>MEPHVLGAVLYWLLLPCALLAACLLRFSGLSLVYLLFLLLLPWFPGPTRCGLQGHTGRLLRALLGLSLLFLVAHLALQICLHIVPRLDQLLGPSCSRWETLSRHIGVTRLDLKDIPNAIRLVAPDLGILVVSSVCLGICGRLARNTRQSPHPRELDDDERDVDASPTAGLQEAATLAPTRRSRLAARFRVTAHWLLVAAGRVLAVTLLALAGIAHPSALSSVYLLLFLALCTWWACHFPISTRGFSRLCVAVGCFGAGHLICLYCYQMPLAQALLPPAGIWARVLGLKDFVGPTNCSSPHALVLNTGLDWPVYASPGVLLLLCYATASLRKLRAYRPSGQRKEAAKGYEARELELAELDQWPQERESDQHVVPTAPDTEADNCIVHELTGQSSVLRRPVRPKRAEPREASPLHSLGHLIMDQSYVCALIAMMVWSITYHSWLTFVLLLWACLIWTVRSRHQLAMLCSPCILLYGMTLCCLRYVWAMDLRPELPTTLGPVSLRQLGLEHTRYPCLDLGAMLLYTLTFWLLLRQFVKEKLLKWAESPAALTEVTVADTEPTRTQTLLQSLGELVKGVYAKYWIYVCAGMFIVVSFAGRLVVYKIVYMFLFLLCLTLFQVYYSLWRKLLKAFWWLVVAYTMLVLIAVYTFQFQDFPAYWRNLTGFTDEQLGDLGLEQFSVSELFSSILVPGFFLLACILQLHYFHRPFMQLTDMEHVSLPGTRLPRWAHRQDAVSGTPLLREEQQEHQQQQQEEEEEEEDSRDEGLGVATPHQATQVPEGAAKWGLVAERLLELAAGFSDVLSRVQVFLRRLLELHVFKLVALYTVWVALKEVSVMNLLLVVLWAFALPYPRFRPMASCLSTVWTCVIIVCKMLYQLKVVNPQEYSSNCTEPFPNSTNLLPTEISQSLLYRGPVDPANWFGVRKGFPNLGYIQNHLQVLLLLVFEAIVYRRQEHYRRQHQLAPLPAQAVFASGTRQQLDQDLLGCLKYFINFFFYKFGLEICFLMAVNVIGQRMNFLVTLHGCWLVAILTRRHRQAIARLWPNYCLFLALFLLYQYLLCLGMPPALCIDYPWRWSRAVPMNSALIKWLYLPDFFRAPNSTNLISDFLLLLCASQQWQVFSAERTEEWQRMAGVNTDRLEPLRGEPNPVPNFIHCRSYLDMLKVAVFRYLFWLVLVVVFVTGATRISIFGLGYLLACFYLLLFGTALLQRDTRARLVLWDCLILYNVTVIISKNMLSLLACVFVEQMQTGFCWVIQLFSLVCTVKGYYDPKEMMDRDQDCLLPVEEAGIIWDSVCFFFLLLQRRVFLSHYYLHVRADLQATALLASRGFALYNAANLKSIDFHRRIEEKSLAQLKRQMERIRAKQEKHRQGRVDRSRPQDTLGPKDPGLEPGPDSPGGSSPPRRQWWRPWLDHATVIHSGDYFLFESDSEEEEEAVPEDPRPSAQSAFQLAYQAWVTNAQAVLRRRQQEQEQARQEQAGQLPTGGGPSQEVEPAEGPEEAAAGRSHVVQRVLSTAQFLWMLGQALVDELTRWLQEFTRHHGTMSDVLRAERYLLTQELLQGGEVHRGVLDQLYTSQAEATLPGPTEAPNAPSTVSSGLGAEEPLSSMTDDMGSPLSTGYHTRSGSEEAVTDPGEREAGASLYQGLMRTASELLLDRRLRIPELEEAELFAEGQGRALRLLRAVYQCVAAHSELLCYFIIILNHMVTASAGSLVLPVLVFLWAMLSIPRPSKRFWMTAIVFTEIAVVVKYLFQFGFFPWNSHVVLRRYENKPYFPPRILGLEKTDGYIKYDLVQLMALFFHRSQLLCYGLWDHEEDSPSKEHDKSGEEEQGAEEGPGVPAATTEDHIQVEARVGPTDGTPEPQVELRPRDTRRISLRFRRRKKEGPARKGAAAIEAEDREEEEGEEEKEAPTGREKRPSRSGGRVRAAGRRLQGFCLSLAQGTYRPLRRFFHDILHTKYRAATDVYALMFLADVVDFIIIIFGFWAFGKHSAATDITSSLSDDQVPEAFLVMLLIQFSTMVVDRALYLRKTVLGKLAFQVALVLAIHLWMFFILPAVTERMFNQNVVAQLWYFVKCIYFALSAYQIRCGYPTRILGNFLTKKYNHLNLFLFQGFRLVPFLVELRAVMDWVWTDTTLSLSSWMCVEDIYANIFIIKCSRETEKKYPQPKGQKKKKIVKYGMGGLIILFLIAIIWFPLLFMSLVRSVVGVVNQPIDVTVTLKLGGYEPLFTMSAQQPSIIPFTAQAYEELSRQFDPQPLAMQFISQYSPEDIVTAQIEGSSGALWRISPPSRAQMKRELYNGTADITLRFTWNFQRDLAKGGTVEYANEKHMLALAPNSTARRQLASLLEGTSDQSVVIPNLFPKYIRAPNGPEANPVKQLQPNEEADYLGVRIQLRREQGAGATGFLEWWVIELQECRTDCNLLPMVIFSDKVSPPSLGFLAGYGIMGLYVSIVLVIGKFVRGFFSEISHSIMFEELPCVDRILKLCQDIFLVRETRELELEEELYAKLIFLYRSPETMIKWTREKE[3x];>MSGAGEALAPGPVGPQRVAEAGGGQLGSTAQGKCDKDNTEKDITQATNSHFTHGEMQDQSIWGNPSDGELIRTQPQRLPQLQTSAQVPSGEEIGKIKNGHTGLSNGNGIHHGAKHGSADNRKLSAPVSQKMHRKIQSSLSVNSDISKKSKVNAVFSQKTGSSPEDCCVHCILACLFCEFLTLCNIVLGQASCGICTSEACCCCCGDEMGDDCNCPCDMDCGIMDACCESSDCLEICMECCGICFPS[3x]

PIEZO channels transmit mechanical force signals to cells, allowing them to make critical decisions during development and in pathophysiological conditions. Here, we report several near-atomic resolution cryo-EM structures of fast-inactivating wild-type human PIEZO1 (hPIEZO1) and its slow-inactivating channelopathy mutants with or without its auxiliary subunit MDFIC. Each hPIEZO1 subunit has a curved blade structure, and the three subunits form the trimeric PIEZO channel, exhibiting a bowl-like shape. MDFIC, a MyoD family inhibitor protein, has recently been identified as an auxiliary subunit of piezo channels capable of decelerating channel inactivation and attenuating channel mechanosensitivity.

The curving effect of MDFIC on hPIEZO1 further encouraged us to test if it can stabilize the unstable channelopathy mutants hPIEZO1-A1988V, hPIEZO1-E756del, and hPIEZO1-R2456H. Indeed, electrophysiological studies showed that co-expression of these channelopathy mutants with MDFIC resulted in significantly reduced mechanosensitivity and inactivation rate. We then co-expressed these hPIEZO1 mutants with MDFIC in HEK293F suspension cells and purified the resulting complex using the same method. Surprisingly, with standard cryo-EM analysis, we obtained high-quality 2D class averages for hPIEZO1-A1988V-MDFIC and hPIEZO1-E756del-MDFIC. Cryo-EM density maps were obtained for hPIEZO1-A1988V-MDFIC and hPIEZO1-E756del-MDFIC with overall resolutions of 3.1 and 2.8 Å, respectively (Figure 4—figure supplements 4 and 5). The densities of the multi-lipidated C-terminal amphipathic helix of MDFIC are clearly present in both the hPIEZO1-A1988V-MDFIC and hPIEZO1-E756del-MDFIC maps. We were surprised to find an apparent lipid density in wild-type hPIEZO1-MDFIC, hPIEZO1-A1988V-MDFIC, and even more evident in the 2.8 Å resolution map of hPIEZO1-E756del-MDFIC in the pore module, where one of its hydrophobic fatty acid tails inserts into the hydrophobic pore formed by I2447, V2450, and F2454, thus sealing the pore to prevent ion flow. Even more surprisingly, the hydrophilic phosphate head interacts directly with R2456, a residue with the more severe form of GOF mutation, on the side of the IH of the pore. In addition, another fatty acid chain of the pore lipid interacts with the acyl chains of the covalently linked MDFIC lipids, forming a stable hPIEZO1-multi-lipidated MDFIC-pore lipid complex.> MDNEKKLFLKALKKKFEGEDPEEKSTNFYCFGGWEQSERKREFTEYAKKAAEKRGGIPFYNPDIGVPLGQRKLMAYRVSGTDAYVEGDDLHFVNNAAIQQMVDDIKRTVIVGMDTAHAVLEKRLGVEVTPETINEYMEVINHALPGGAVVQEHMVEVHPGIVEDCYAKVFTGDDNLADE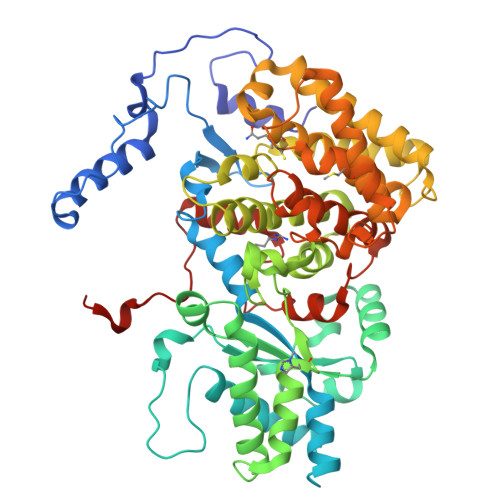LDKRILIDINKEFPEEQAEQLKSYIGNRTYQVNRVPTIVVRACDGGTVSRWSAMQIGMSFISAYKLCAGEAAIADFSFAAKHADVIEMGTIMPARRARGPNEPGGVAFGTFADIVQASRVSDDPANVSLEVIAGAAALYDQVWLGSYMSGGVGFTQYATAAYTDDILDDFLYYGMEYVEDKFGICGSEPTMDVVRDISTEVTLYSLEQYEEYPTLLEDHFGGSQRAAVAAAAAGCSTAFATGNSNAGVNGWYLSQILHKEAHSRLGFYGYDLQDQCGASNSLSIRSDEGLIHELRGPNYPNYAMNVGHQPEYAGIAQAPHAARGDAFCTNPLIKVAFADKDLSFDFTSPRKSIAKGALREFIPEGERDLIIPAGK> MLPPDILQNGEFETIYFQTNPTYIKSPIHIPKSTIGKPDTVKIRHFFALLHQDLVVLGLEVFVYLQIYSDFVEKYVYVSKCDTVGLEKSTIKIGKVIGPVLQYIINYNGYKIKMKNLDEKSKDLSDPSTLVRLQRLRDKLPDIYPNLPYYNDIPPKEECIEYRTLPKTQNLRLCVFTKPAKEYLFPNSAKNPYKNLLNGQSLLRAWISIIDSITKGWNNHKLMIPGADKYATRKFIEKYSDWSEGHIFKKDGLAVQAIPLFPDDPKGRFLELVIVECRYGKMTVSRFYQELAYRQEFLLGDCVSLIGCCKENLEVTYHDD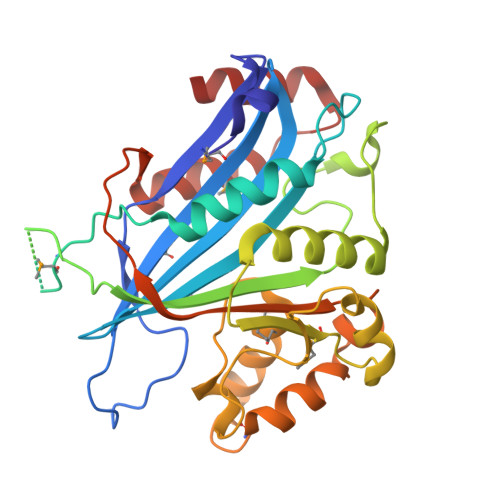LVSTVTISEYKEFMNLLKLVDFSDRVEVSNFVSNYRKSK>[4x]AELLLGVNIDHIATLRNARGTAYPDPVQAAFIAEQAGADGITVHLREDRRHITDRD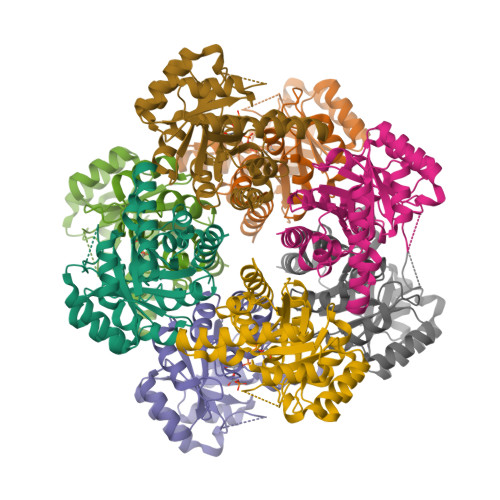VRILRQTLDTRMNLEMAVTEEMLAIAVETKPHFCCLVPEKRQEVTTEGGLDVAGQRDKMRDACKRLADAGIQVSLFIDADEEQIKAAAEVGAPFIEIHTGCYADAKTDAEQAQELARIAKAATFAASLGLKVNAGHGLTYHNVKAIAAIPEMHELNIGHAIIGRAVMTGLKDAVAEMKRLMLEARG> MGSDKIHHHHHHMKYIINHSNDTAFNIALEEYAFKHLLDEDQIFLLW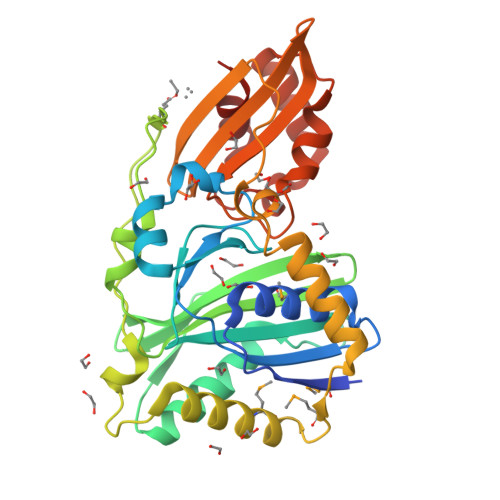INKPSIIVGRHQNTIEEINRDYVRENGIEVVRRISGGGAVYHDLNNLNYTIISKEDENKAFDFKSFSTPVINTLAQLGVKAEFTGRNDLEIDGKKFCGNAQAYINGRIMHHGCLLFDVDLSVLANALKVSKDKFESKGVKSVRARVTNIINELPKKITVEKFRDLLLEYMKKEYPEMTEYVFSEEELAEINRIKDTKFGTWDWNYGKSPEFNVRRGIKFTSGKVEVFANVTESKIQDIKIYGDFFGIEDVAAVEDVLRGVKYEREDVLKALKTIDITRYFAGISREEIAEAVVG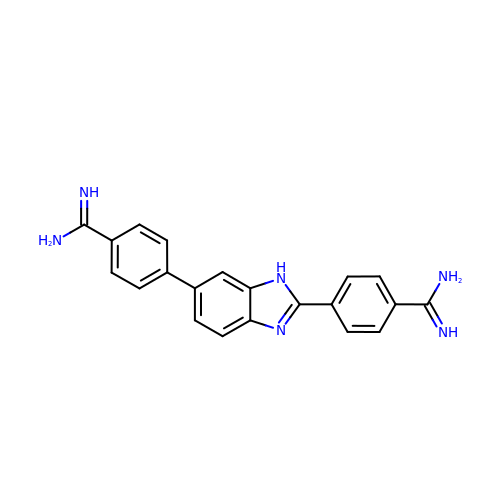4,4'-(1H-benzimidazole-2,6-diyl)di(benzene-1-carboximidamide) | C21 H18 N6 | PHJDIHHRXDMKMB-UHFFFAOYSA-N The enzyme CdaA, which synthesizes an essential second messenger cyclic di-AMP (c-di-AMP) in many pathogenic bacteria, has emerged as a promising candidate for the development of novel antibiotics. Additionally, c-di-AMP regulates the bacterial stringent response, further underscoring its significance. The synthesis of c-di-AMP is mediated by enzymes possessing a diadenylate-cyclase (DAC) domain.

Recently, we performed an in silico design of an L. monocytogenes CdaA inhibitor (Compound 7) that binds to LmCdaA in the micromolar range with a dissociation constant (Kd) approximately eight times lower than that of ATP. This bithiazole ring compound, which is distinct from adenosine, binds in the same position and thus serves as a promising lead compound for further optimization. The reported structure of BsCdaA in complex with an inhibitor (Compound 7) originally developed for LmCdaA, which reveals an identical ligand-binding mode, provides structural evidence supporting the efficacy of this approach.

>[2x]GPTPVEEAQQKTIEAITKAINYMAKRRIGALLTIERDTGMGDYIETGIPLNAKVSSELLINIFIPNTPLHDGAVIMKNNEIAAAACYLPLSESPFISKELGTRHRAAVGISEVTDSLTIIVSEETGGVSVAKNGDLHRELTEEALKEMLEAEFKK>[2x]GSGIM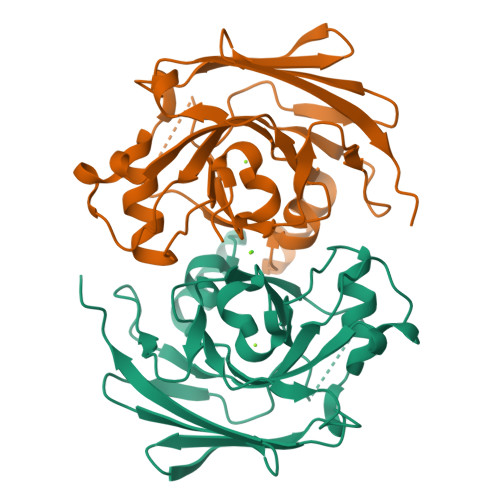AASRPLSRFWEWGKNIVCVGRNYADHVREMRSAVLSEPVLFLKPSTAYAPEGSPILMPAYTRNLHHELELGVVMGKRCRAVPEAAAMDYVGGYALCLDMTARDVQDECKKKGLPWTLAKSFTASCPVSAFVPKEKIPDPHKLKLWLKVNGELRQEGETSSMIFSIPYIISYVSKIITLEEGDIILTGTPKGVGPVKENDEIEAGIHGLVSMTFKVEKPEY>[4x]KVTLPDL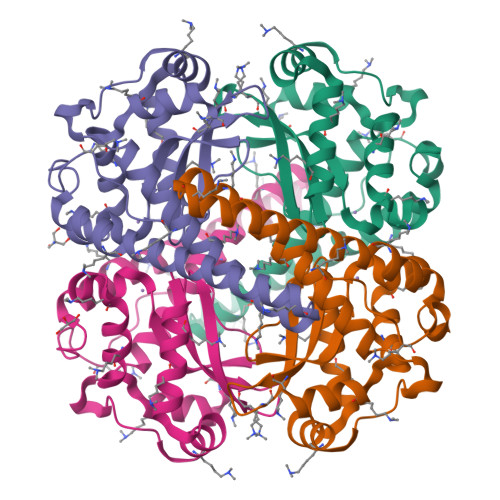KWDFGALEPYISGQINELHYTKHHQTYVNGFNTAVDQFQELSDLLAKEPSPANARKMIAIQQNIKFHGGGFTNHCLFWENLAPESQGGGEPPTGALAKAIDEQFGSLDELIKLTNTKLAGVQGSGWAFIVKNLSNGGKLDVVQTYNQDTVTGPLVPLVAIDAWEHAYYLQYQNKRPDYFKAIWNVVNWKEASRRFDAGKI>[2x]GAGAGAGAGAGMARHFVLNTGAKIPSVGLGTWQSDPGVVGDAVYTAVKAGYRHIDCAKVYGNEKEIGLALKKLFEEGVVKREDLFITSKLWNDRHAPEDVPEALNESLTDLQLDYLDLYLIHWPFR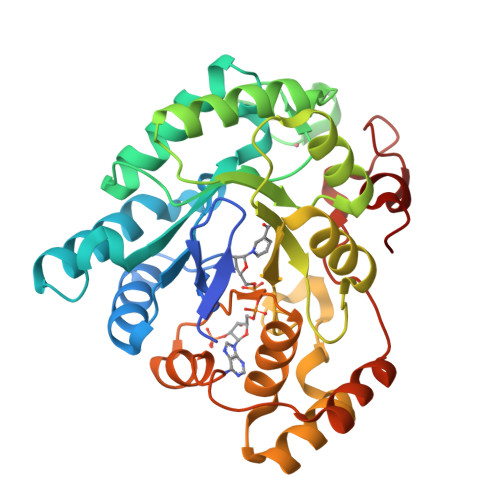VKKGTNTSPENFITPDIPATWGAMEKCYDAGKARAIGVSNFSSKKLGDLLAVARVHPAVDQVECHPGWQQTKLHNFCQSTGVHLTAYSPLGSPGTTWMNGNVLKEPVIISIAEKLGKTPAQVALRWNIQMGHSVLPKSTNEERIKQNLDVYDWSIPDDLLAKFSEIKQARLLRGNFIVNPQSVYKTHEELWDGEL> MTHHHHHHAMALTDRGMTYDLDPKDGSSAATKPVLEVTKKVFDTAADAAGQTVTVEFKVSGAEGKYATTGYHIYWDERLEVVATKTGAYAKKGAALEDSSLAKAENNGNGVFVASGADDDFGADGVMWTVELKVPADAKAGDVYPIDVAYQWDPSKGDLFTDNKDSAQGKLMQAYFFTQGIKSSSNPSTDEYLVKANATYADGYIAIKAGEP;> MGSSNTVTSAVKTQYVE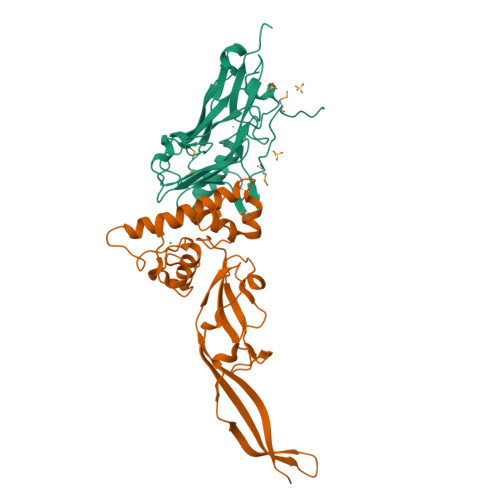IESVDGFYFNTEDKFDTAQIKKAVLHTVYNEGYTGDDGVAVVLREYESEPVDITAELTFGDATPANTYKAVENKFDYEIPVYYNNATLKDAEGNDATVTVYIGLKGDTDLNNIVDGRDATATLTYYAATSTDGKDATTVALSPSTLVGGNPESVYDDFSAFLSDVKVDAGKELTRFAKKAERLIDGRDASSILTFYTKSSVDQYKDMAANEPNKLWDIVTGDAEEE> GPLSVAPEMDIMDYCKKEWRGNTQKATCMKMGYEEVSQKFTSIRRVRGDNYCALRATLFQAMSQAVGLPPWLQDPELMLLPEKLISKYNWIKQWKLGLKFDGKNEDLVDKIKESLTLLRKKWAGLAEMRTAEARQIACDELFTNEAEEYSLYEAVKFLMLNRAIELYNDKEKGKEVPFFSVLLFARDTSNDPGQLLRNHLNQVGHTGGLEQVEMFLLAYAVRHTIQVYRLSKYNTEEFITVYPTDPPKDWPVVTLIAEDDRHYNIPVRVCEETSL

Here, we reveal a previously unannotated human DUB, OTULIN (also known as FAM105B), which is exquisitely specific for Met1 linkages. FAM105B comprises 352 amino acids (aa), and the OTU domain spans the majority of the protein (aa 80–352) and an N-terminal region with predicted helical content. Having established FAM105B as a Met1-linkage-specific OTU DUB, we named the enzyme OTULIN (OTU DUB with linear linkage specificity). Crystal structures of the OTULIN catalytic domain in complex with diubiquitin reveal Met1-specific Ub-binding sites and a mechanism of substrate-assisted catalysis in which the proximal Ub activates the catalytic triad of the protease.

OTULINcat was crystallized, and its structure was determined to 1.3 Å resolution with SeMet phasing. OTULINcat adopts an OTU fold most similar to OTUB1 (root-mean-square deviation [rmsd] 2.1 Å, DALI Z score 8.7). Interestingly, catalytic triad residues His339 and Cys129 display two alternate conformations. In the “active” conformation (occupancy ∼30%), the catalytic triad is formed by interactions between Asn341, His339, and Cys129; e.g., as observed in OTUB1 in complex with Ub suicide inhibitor (Wiener et al., 2012). In the “inhibited” conformation (occupancy ∼70%), Asp336 pulls His339 away from its catalytic position, and Cys129 flips to an inactive rotamer. Linkage specificity in DUBs is not well understood, and the structure of apo OTULIN did not explain its Met1 specificity, because of its structural similarity to the Lys48-specific OTUB1. Ub-based suicide inhibitors that comprise an electrophilic group at the Ub C terminus (Borodovsky et al., 2002) covalently modify most OTU domain DUBs but showed no reactivity against FAM105B.3-[1-[[4-(pyrrolidin-1-ylmethyl)phenyl]methyl]indol-6-yl]-1~{H}-pyrazol-5-amine | C23 H25 N5 | 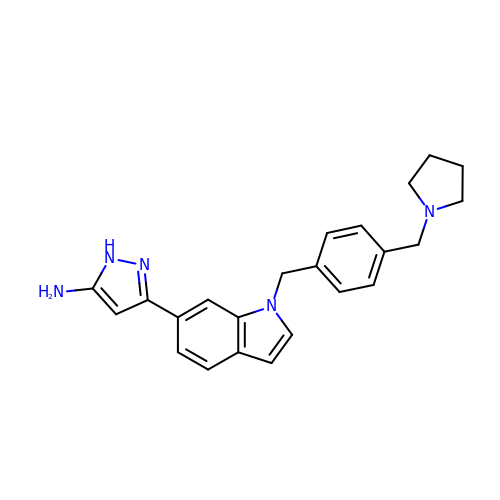QHKSDDZUHNXXME-UHFFFAOYSA-N> MAHHHHHHVGTDLTDFRVATWNLQGASATTESKWNINVRQLISGENAVDILAVQEAGSPPSTAVDTGRVIPSPGIPVRE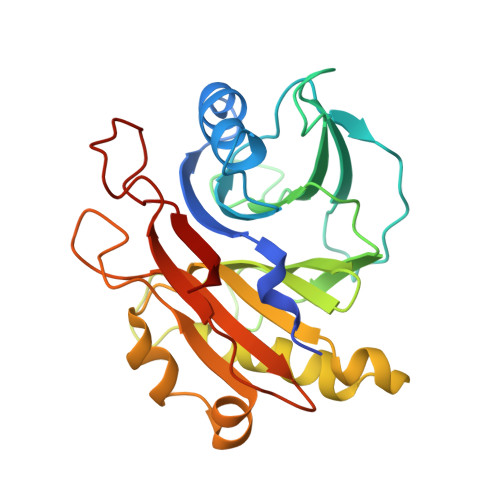LIWNLSTNSRPQQVYIYFSAVDALGGRVNLALVSNRRADEVFVLSPVRQGGRPLLGIRIGNDAFFTAHAIAMRNNDAPALVEEVYNFFRDSRDPVHQALNWMILGDFNREPADLEMNLTVPVRRASEIISPAAATQTSQRTLDYAVAGNSVAFRPSPLQAGIVYGARRTQISSDHFPVGVSRR> GTAGLPRRIIKETQRLLAEPVPGIKAEPDESNARYFHVVIAGPQDSPFEGGTFKLELFLPEEYPMAAPKVRFMTKIYHPNVDKLGRICLDILKDKWSPALQIRTVLLSIQALLSAPNPDDPLANDVAEQ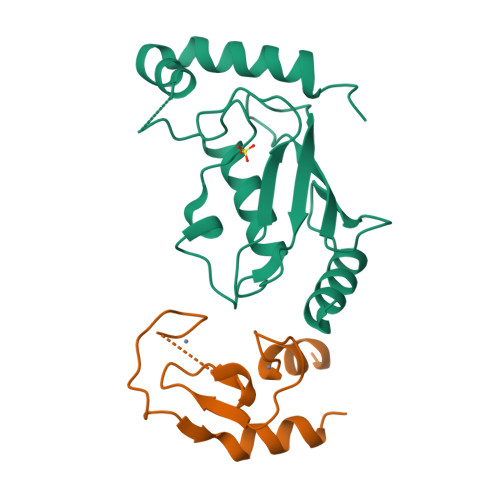WKTNEAQAIETARAWTRLYAMNNI;> GSASGILLNVKEEVTCPICLELLTEPLSLHCGHSFCQACITANHKKSMLYKEGERSCPVCRISYQPENIQPNRHVANIVEKLREVKLSPEEGQ>[2x]MPPRKELVGNKWFIENYENETESLVIDANKDESIFIGKCSQVLVQIKGKVNAISLSETESCSVVLDSSISGMDVIKSNKFGIQVN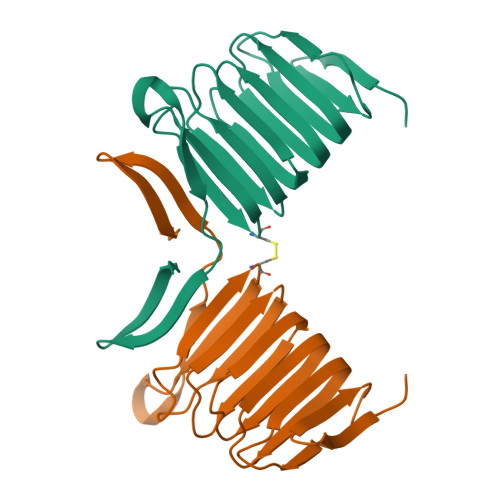HSLPQISIDKSDGGNIYLSKESLNTEIYTSCSTAINVNLPIGEDDDYVEFPIPEQMKHSFADGKFKSAVFEHAG4-{[(2-amino-4-oxo-3,4-dihydropteridin-6-yl)methyl]amino}benzoic acid | C14 H12 N6 O3 | 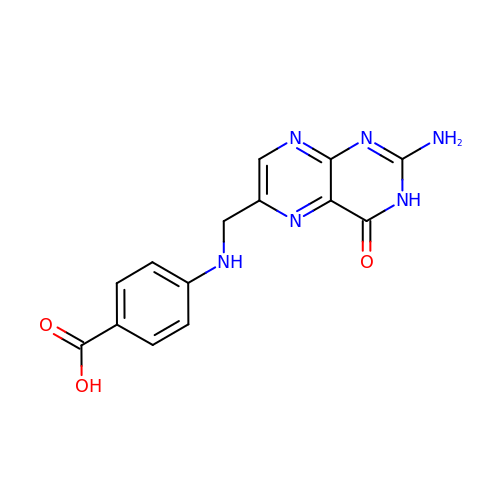JOAQINSXLLMRCV-UHFFFAOYSA-N>TSNVITQDLPIPVASRGFADIVGFGLDGVVIGRNAVNLQPFLAVKNFAQNAGGWLTTKHVRLIADTTGTGKGDIVGFGNAGVYVSVNNGKNTFADPPKMVIANFGYDAGGWRVEKHLRYLADIRKTGRADIIGFGEKGVLVSRNNGGLNFGPATLVLKDFGYDAGGWRLDRHLRFLADVTGNGHLDIVGFGDKHVFISRNNGDGTFAPAKSVIDNFCIDAGGWKIGDHPRFVADLTGDGTADIIGCGKAGCWVALNNGGGVFGQVKLVINDFGTDKGWQAAKHPRFIADLTGNGRGDVVGFGNAGVYVALNNGDGTFQSAKLVLKDFGVQQGWTVSKHRRFVVDLTGDGCADIIGFGEKETLVSYNDGKGNFGPVKALTNDFSFSGGKWAPETTVCWMANLDSSRH[2x]

In this paper, we report the crystal structures of a lectin from Agrocybe aegerita, designated as AAL2, in its apo- and complex forms with GlcNAc and GlcNAcβ1-3Galβ1-4GlcNAc, as part of our endeavors to develop a system to facilitate the identification and purification of O-GlcNAcylated proteins. AAL2 was recently discovered from the fruit body of the edible mushroom A. aegerita. AAL2 was found to specifically bind nonreducing terminal N-acetylglucosamine (GlcNAc) moieties of either alpha- or beta-linkage and was reported to have the activity of inducing apoptosis in hepatoma cells in vitro as well as inhibiting hepatoma growth in tumour-bearing mice in vivo. The overall structure of AAL2 monomer is a single domain with the shape of cylindrical torus with a diameter of about 51Å and a height of about 27Å, showing a very regular, seven-bladed β-propeller fold formed by the blades packing in a circular array.

The structures of AAL2, AAL2-GlcNAc and AAL2-GlcNAcβ1-3Galβ1-4GlcNAc were determined at resolutions of 2.0Å, 2.1Å, and 2.0Å, respectively. There are two virtually identical AAL2 monomers arranged around a two-fold pseudoaxis of symmetry in an asymmetric unit in both the structures of AAL2 and AAL2-GlcNAc, and one AAL2 monomer in AAL2-GlcNAcβ1-3Galβ1-4GlcNAc, while the protein exists as monomers in solution as determined from its elution volume on a Superdex 200 10/300 GL column. The structure of AAL2-GlcNAc complex revealed six binding sites out of the seven W-motifs, with the exception of motif WI. Glycan ligands are bound in shallow pockets located on the entrance side, between the connecting segment and the 2–3 loop of each W-motifs (except for WI). The binding pocket for GlcNAc consists of two parts. The major part is formed by the segment connecting WII and WIII, including the side chains of Asn104, Trp112 and His117 and main chain atoms of Gly110 and Gly111. The other part is formed by the main chain atoms of Gly136, Glu137, and Lys138 from the 2–3 loop of WIII. With the presence of both the polar and hydrophobic interactions, GlcNAc is bound tightly in the shallow pocket formed on the protein surface, with the head of N-acetyl group buried inside the pocket and the reduced O1 as well as O6 hydroxyl pointing outside into the solvent region. In addition to glycans, AAL2 also binds two cations per molecule as observed in the structure of AAL2-GlcNAc complex. Similar metal ion binding properties were also observed for PVL. These cations are located in the 1–2 loops of WV and WVII of AAL2, where highly negatively-charged cages are formed.>MIKRPIELSHDFLSQVLDKNSIAIDATMGNGNDTVFLSHLAKKVYAFDVQEQALIKTREKLEQLNIKNVQLILDGHQTINKYVTEPIRAAIFNLGYLPSADKSVITQPATTLTAIKKILERLEIGGRLAIMVYYGHEGGDKEKDAVLNFVKELDQQHFTVMLYQPLNQIN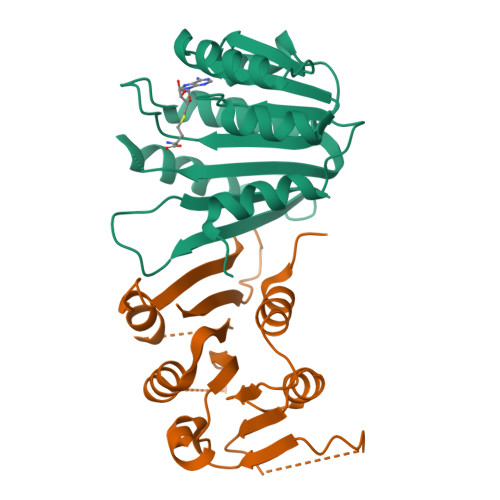TPPFLVMIEKL[2x]> MAVAA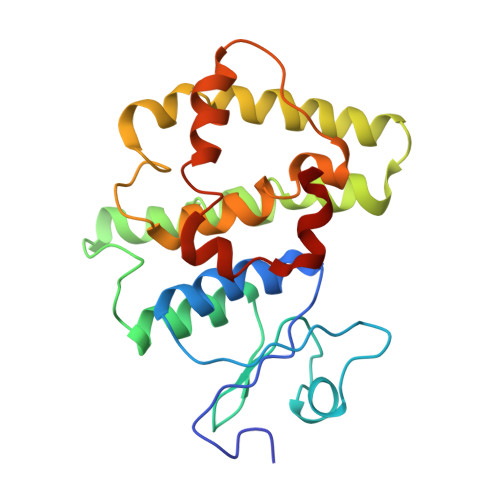NKRSVMTLFSGPTDIYSHQVRIVLAEKGVSFEIEHVEKDNPPQDLIDLNPNQSVPTLVDRELTLWESRIIMEYLDERFPHPPLMPVYPVARGESRLYMHRIEKDWYTLMNTIINGSASEADAARKQLREELLAIAPVFGQKPYFLSDEFSLVDCYLAPLLWRLPQLGIEFSGPGAKELKGYMTRVFERDSFLASLTEAEREMRLGRS> AQSVPYGVSQIKAPALHSQGYTGSNVKVAVIDSGIDSSHPDLKVAGGASMVPSETNPFQDNNSHGTHVAGTVAALNNSIGVLGVAPSASLYAVKVLGADGSGQYSWIINGIEWAIANNMDVINMSLGGPSGSAALKAAVDKAVASGVVVVAAAGNEGTSGSSSTVGYPGKYPSVIAVGAVDSSNQRASFSSVGPELDVMAPGVSIQSTLPGNKYGAYNGTSMASPHVAGAAALILSKHPNWTNTQVRSSLENTTTKLGDSFYYGKGLINVQAAAQ;> YAPSALVLTVGKGVSATTAAPERAVTLTCAPGPSGTHPAAGSACADLAAVGGDLNALTRGEDVMCPKVYDPVLLTVDGVWQ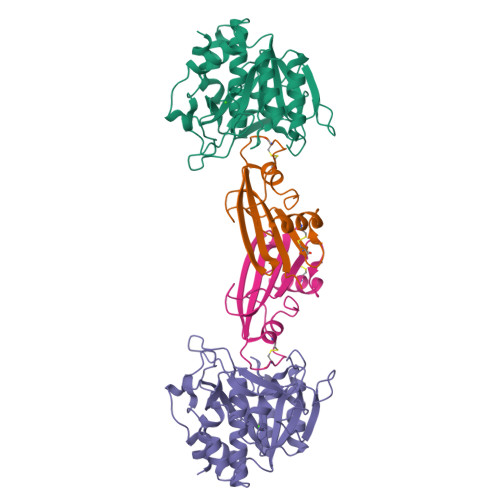GKRVSYERVFSNECEMNAHGSSVFAF>ASTLKSGSKEVENLKKPFMPPREVHVQVTHSMPPQKIEIFKSLDNWAEENILVHLKPVEKCWQPQDFLPDPASDGFDEQVRELRERAKEIPDDYFVVLVGDMITEEALPTYQTMLNTLDGVRDETGASPTSWAIWTRAWTAEENRHGDLLNKYLYLSGRVDMRQIEKTIQYLIGSGMDPRTENSPYLGFIYTSFQERATFISHGNTARQAKEHGDIKLAQICGTIAADEKRHETAYTKIVEKLFEIDPDGTV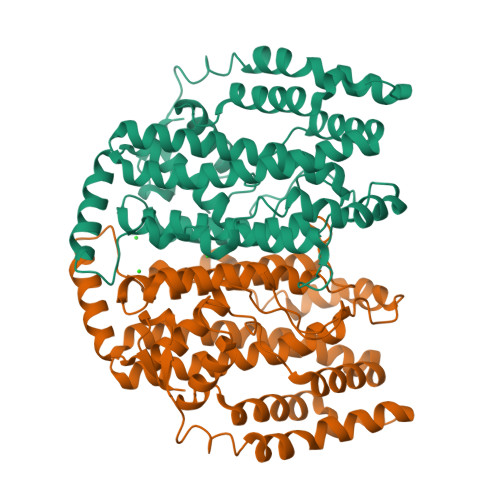LAFADMMRKKISMPAHLMYDGRDDNLFDHFSAVAQRLGVYTAKDYADILEFLVGRWKVDKLTGLSAEGQKAQDYVCRLPPRIRRLEERAQGRAKEAPTMPFSWIFDRQVKL[6x]Here we describe extendable linear, curved and angled protein building blocks, as well as inter-block interactions, that conform to specified geometric standards; assemblies designed using these blocks inherit their extendability and regular interaction surfaces, enabling them to be expanded or contracted by varying the number of modules, and reinforced with secondary struts. We construct twistless helix repeat (THR) protein blocks from identical straight α-helices (typically 2–4 helices in each unit); the length of the blocks can be varied simply by varying the number of repeat units. Restricting helical geometry to ideal straight helices with zero helical twist in principle considerably limits what types of structure could be built, but this is more than compensated by the great simplification of downstream material design, as illustrated below. Using X-ray crystallography and electron microscopy, we validate nanomaterial designs ranging from simple polygonal and circular oligomers that can be concentrically nested, up to large polyhedral nanocages and unbounded straight ‘train track’ assemblies with reconfigurable sizes and geometries that can be readily blueprinted.

To generate straight, linear THRs, we set Δθ to zero. This results in perfectly straight repeat proteins in which each repeat unit is translated but not rotated relative to the previous unit. We tested 33 linear THRs (with Δh = 0) with helices either about 20 or about 40 residues in height; 23 of 33 tested designs were solubly expressed, and 13 of 19 designs analysed by SEC were primarily monomeric as designed. Structural characterization of the linear building blocks by X-ray crystallography individually and/or cryogenic EM (cryo-EM) in the context of assemblies (see below) revealed that both the detailed internal structures and the overall straight linear geometry were successfully achieved.

>PKKIVKDAKEKLEKLLEDAKDGGEELALDIAEELAREAEKALKELLREGASPELIVDLAETALRALLEIAKDGGEELALDIARILAKLAEVALEVLLKDGASPKLIVDLAKTALRALLEIAEDGGEELALDIAEILAELAEVALRVLLKDGASPKLIEDLAKTALDALEEIARDGGEELAEDIDRILRKLEKVARDVLRKDGAS[2x]> IESIIKTATDTVKSEINAELGVVPSLNAVETGATSNTEPEEAIQTRTVINQHGVSETLVENFLSRAALVSKRSFEYKDHTSSAAQTDKNFFKWTINTRSFVQLRRKLELFTYLRFDAEITILTTVAVNGSSNNTYMGLPNLTLQAMFVPTGALTPEKQDSFHWQSGSNASVFFKISDPPARMTIPFMCINSAYSVFYDGFAGFEKSGLYGINPADTIGNLCVRIVNEHQPVGFTVTVRVYMKPKHIKAWAPRPPRTLPYMSIANANYKGKKRAPNALNAIIGNRDSVKTMPHNIVTT;> GVPTYLLPGSGQFLTTDDHSSAPVLPCFNPTPEMHIPGQVRNMLEVVQVESMMEINNTESAVGMERLKVDISALTDVDQLLFNIPLDIQLDGPLRNTLVGNISRYYTHWSGSLEMTFMFCGSFMATGKLILCYTPPGGSCPTTRETAMLGTHIVWDFGLQSSVTLIIPWISGSHYRMFNNDAKSTNANVGYVTCFMQTNLIVPSESSDTCSLIGFIAAKDDFSLRLMRDSPDIGQIDHLHAAEAAYQ;> SPSAEACGYSDRVLQLKLGNSAIVTQEAANYCCAYGEWPNYLPDHEAVAIDKPTQPETATDRFYTLKSVKWEAGSTGWWWKLPDALNNIGMFGQNVQHHYLYRSGFLIHVQCNATRFHQGALLVVAIPEHQRGAHNTNTSPGFDDIMKGEEGGTFNHPYVLDDGTSLACATIFPHQWINLRTNNSATIVLPWMNAAPMDFPLRHNQWTLAIIPVVPLGTRTMSSMVPITVSIAPMCCEFNGLRHAITQ;> GAQVTRQQTGTHENANIATNGSHITYNQINFYKDSYAASASKQDFSQDPSKFTEPVVEGLKAGAPVLK

EV-D68 is an atypical enterovirus that usually causes mild respiratory tract disease, but is also associated with severe lower respiratory tract infections and acute flaccid myelitis. Following receptor binding and endocytosis, virus particles uncoat by forming a proteinaceous pore spanning the endosomal membrane through which they eject their genome into the cytosol. In this study, we showed that EV-D68-947 is a dual receptor-binding virus that can use both sialylated glycans and sGAGs as receptors. Structures of EV-D68-947 were determined after incubation of the virus either in the absence of a receptor analogue, with 6′SLN (a sialylated trisaccharide), with dp6 (a heparin-derived hexasaccharide), or with LMWH at 33 °C.

Similarly, EV-D68-947 infection was neutralized by soluble heparan sulfate as well as fondaparinux (sulfated pentasaccharide) and dp6 (a heparin-derived hexasaccharide). We did not observe density corresponding to dp6 or LMWH in the EV-D68-947 structure, either because these ligands, in contrast to Sia, interact with the virus via a multitude of low-affinity and/or transient electrostatic interactions or because the bound ligands do not occupy all icosahedral symmetry related sites. Structural analyses showed that, like 6′SLN, both sGAG analogues induced movements of the VP1 GH loop into the VP1 hydrophobic pocket, causing displacement of the pocket factor, as previously observed. This indicates that both Sia and sGAGs can prime the uncoating process. By contrast, determination of the ratio between the number of EV-D68-947 full and empty particles after 1 h incubation at 33 °C showed that the sGAG analogues dp6 and LMWH, but not 6’SLN, promoted genome release. Unfortunately, we were unable to determine the exact binding site of sGAGs on the EV-D68-947 particle by cryo-EM.>[2x]MAANKSKGQSSLALHKVIMVGSGGVGKSALTLQFMYDEFVEDYEPTKADSYRKKVVLDGEEVQIDILDTAGLEDYAAIRDNYFRSGEGFLLVFSITEHESFTATAEFREQILRVKAEED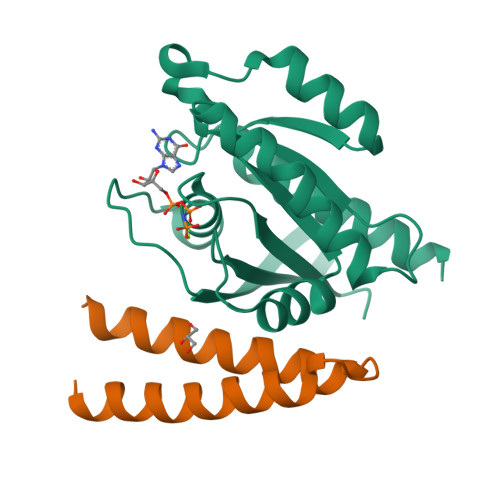KIPLLVVGNKSDLEERRQVPVEEARSKAEEWGVQYVETSAKTRANVDKVFFDLMREIRTKKMSENK;>GPLGSETQAGIKEEIRRQEFLLNSLHRDLQGGIKDLSKEHRLWEVLRILTALRRKLREA[2x]> GPRSMAPTPESDKLKSEGNAAMARKEYSKAIDLYTQALSIAPANPIYLSNRAAAYSASGQHEKAAEDAELATVVDPKYSKAWSRLGLARFDMADYKGAKE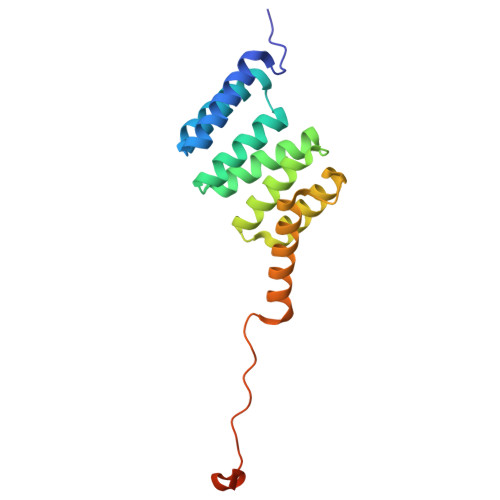AYEKGIEAEGNGGSDAMKRGLETTKRKIEEANRGAEPPADDVDDAAGASRGAGGMPDLSSLASM> MEVYRRIAERVRGALWAHHRRLMPERQFHRILAYVYNNKYEYQIRFDRMSVVGRAWAGRVEVMTTPGG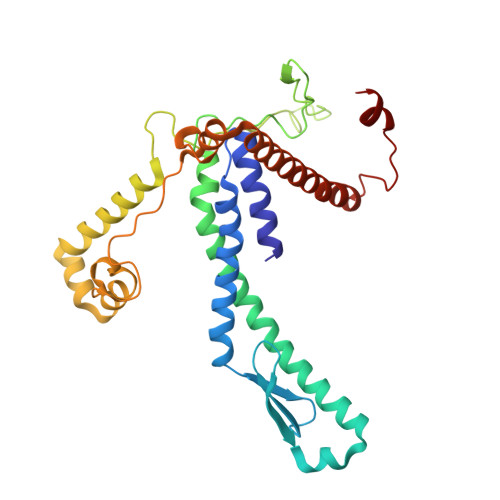FLKRVRVHPAVEDLSPAQQHKLVLAAYADACQQGRALMEQAELKVYKQFLQDLKPIILGIRDNPEFYTVPEDSVETIGGVLRRDQAPLDGGAAANAAGAVHRTIPMARAHQPVDEVRRRHAWEDQWLASKQGQRWAHSLRGKEYFTRHGPQYRPRGAPGAKTRTLPFELLAPYTPMDEGRLLRTNWVAYMDSKHVAESLWTRAKVADREKQLRQLQERGQAWHRPINEDAVQRW> MNYATVNDLCARYTRTRLDILTRPKTADGQPDDAVAE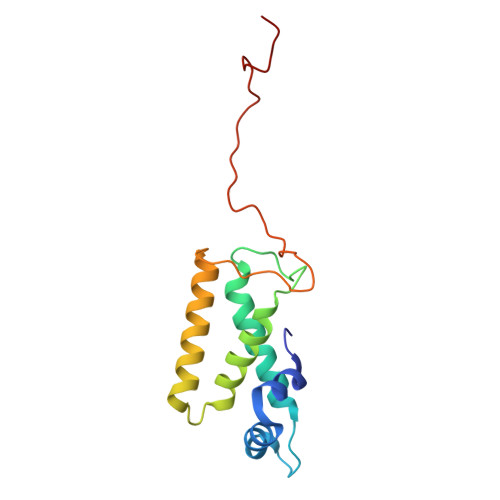QALADASAFIDGYLAARFVLPLTVVPSLLKRQCCVVAWFYLNESQPTEQITATYRDTVRWLEQVRDGKTDPGVESRTAASPEGEDLVQVQSDPPVFSRKQKGFI>[3x]AQVINTFD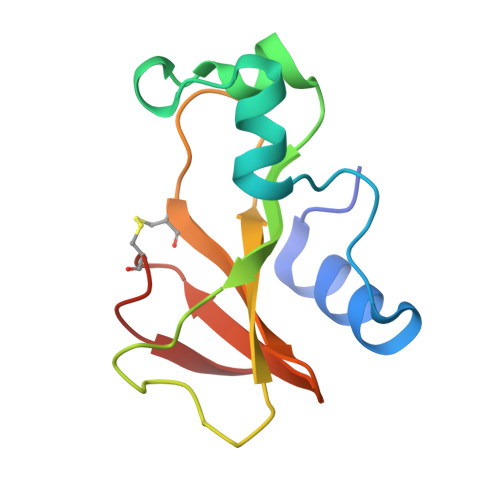GVADYLQTYHKLPDNYITKSEAQALGWVASKGNLADVAPGKSIGGDIFSNREGKLPGKSGRTWREADINYTSGFRNCDRILYSSDWLIYKTTDCYQTFTKIR In purple bacterial photosynthesis, light energy absorbed by light-harvesting 2 (LH2) complex is transferred via the LH1 complex to the reaction center complex, where it is trapped by the primary charge separation reactions. All such complexes are formed by the circular oligomerization of dimer building blocks consisting of pairs of low–molecular weight, hydrophobic apoproteins to which bacteriochlorophyll (BChl) and carotenoid (Car) molecules are noncovalently bound. We report the 2.4 Ångström resolution structure of the light-harvesting 2 (LH2) complex from Marichromatium (Mch.) purpuratum determined by cryogenic electron microscopy. The structure contains a heptameric ring that is unique among all known LH2 structures, explaining the unusual spectroscopic properties of this bacterial antenna complex.

Briefly, 17,338 electron cryomicrograph movies were collected, and 3.05 million particles were picked for data processing. Figure 1 (A to C) shows three views of the cryo-EM map of the Mch. purpuratum LH2 complex at 2.4 Å resolution, which is a previously unidentified, circular LH2 structure formed of seven α/β apoprotein heterodimer subunits. Seven α-apoprotein α helices form an inner ring of 25.4 Å diameter and the seven β-apoprotein α helices form an outer ring of 55.0 Å diameter. The complete α-apoprotein can be traced in the structure apart from the N- and C-terminal amino acids, and the β-apoprotein can be fully traced apart from the first four N-terminal amino acids. Both apoproteins have a single membrane-spanning α helix, with their N termini on the cytoplasmic side of the complex and their C termini on the periplasmic side. Each α/β heterodimer binds, noncovalently, three molecules of BChl a and two molecules of the carotenoid, okenone. Two of the BChl a molecules form a strongly interacting dimer with their Mg2+ atoms liganded by two His residues, α-His49 and β-His38. The third monomeric BChl a molecule is located on the cytoplasmic side of the complex; its Mg2+ atom is liganded to α-Asp21, and there is an H-bond between its C-31 carbonyl group and β-His25 from the β-apoprotein in the next heterodimer. The structure of the LH2 complex from Mch. purpuratum described here is the first direct observation of these two populations of different carotenoids, which serve structurally and spectroscopically distinct BChl a molecules, and it accounts for the spectroscopic properties of these pigments, which have lain unexplained for more than 24 years. The 3.6 Å distance is consistent with the rapid (<200 fs) energy transfer from Car1 to the nearest B828 pigment, and Car2 is precisely positioned, with a distance of 3.2 Å, to transfer its excitation energy to B800. The extended N-terminal domain for LH2α modifies the packing of α/β heterodimers, widening their spacing by 12° and creating space for binding an extra carotenoid.

>MKVPVMMADESIATINHPEDDWKIWTVINPATWMVPFFGILFVQMWLIHSYALSLPGYGFKDSVRVAQPA[7x];>[7x]ADPKAANLSGLTDAQAKEFHEHWKHGVWSWVMIASAVHVVTWIYQPWF>[3x]AQLQNLVLKDREATPNDHTFVPRDIRDN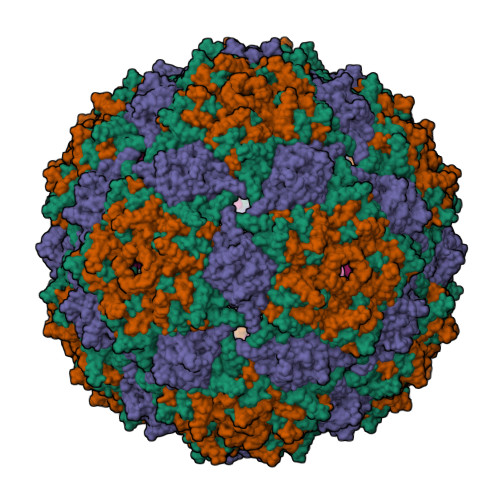VGEVVESTGVPIGESRFTISLRKTSNGRYKSTLKLVVPVVQSQTVNGIVTPVVVRTSYVTVDFDYDARSTTKERNNFVGMIADALKADKMLVHDTIVNLQGVY> GPGSPPGPPTSIHVEEITDTTATLSWRPGPDNHSPITAYTIQA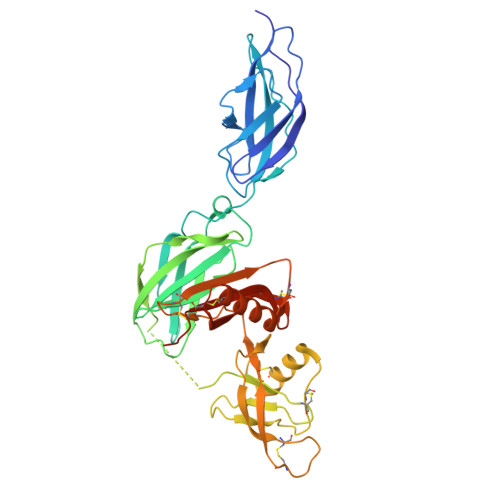RTPFSLGWQAVSTVPEVVGGSHLTATVIELNPWVEYEFRVLASNAVGTGEPSKPSKKARTKDTVPKVTPANVSGGGGSRSELVITWEPVPEELQNGAGFGYVVAFRPFGSTGWMQAAVPSPEASKYVFKNETILPFSPFQVKVGAYNNKGEGPFGPVITIYSAEGGGSGGGSGYIEALAANAGTGFAVAEPQVAMFCGKLNMHINIQTGRWEPDPSGSKTCVGTKEGVLQYCQEIYPELQITNVVEANQPVKIENWCKKDKKQCKGHAHIVVPYKCLVGEFVSDVLLVPEKCKFFHKERMDMCVSHQQWHGVAKEACSKGNMVLHSYGMLLPCGIDKFHGTEYVCCPSTRPEEPAPPASPSKAAA>MITAQAVLYTQHGEPKDVLFTQSFEIDDDNLAPNEVIVKTLGSPVNPSDINQIQGVYPSKPAKTTGFGTTEPAAPCGNEGLFEVIKVGSNVSSLEAGDWVIPSHVNFGTWRTHALGNDDDFIKLPNPAQSKANGKPNGLTINQGATISVNPLTAYLMLTHYVKLTPGKDWFIQNGGTSAVGKYASQIGKLLNFNSISVIRDRPNLDEVVASLKELGATQVITEDQNNSREFGPTIKEWIKQSGGEAKLALNCVGGKSSTGIARKLNNNGLML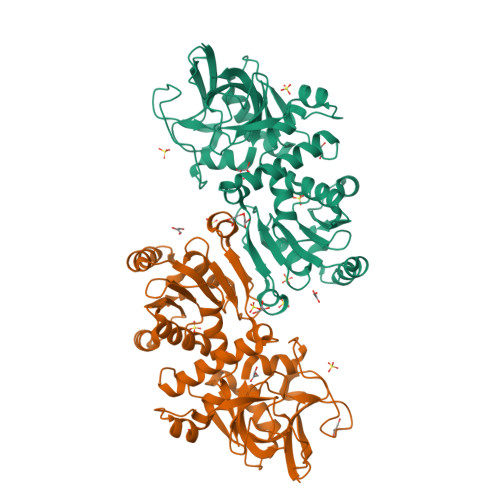TYGGMSFQPVTIPTSLYIFKNFTSAGFWVTELLKNNKELKTSTLNQIIAWYEEGKLTDAKSIETLYDGTKPLHELYQDGVANSKDGKQLITY[2x]>SNAMNDTPDDTFVSGYLLYLLAASSEEASAQFHDHIRAQGLRVPEWRVLACLVDNDAMMITRLA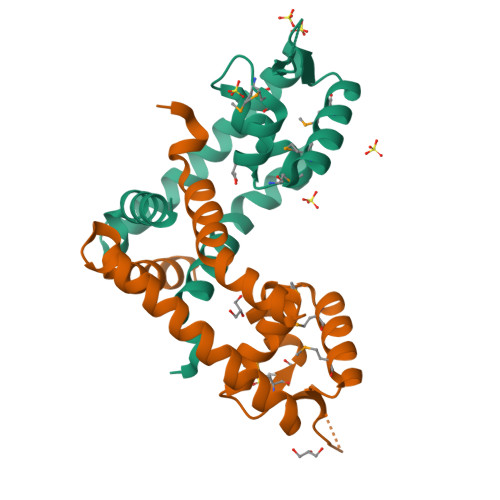KLSLMEQSRMTRIVDQMDARGLVTRVADAKDKRRVRVRLTDDGRALAESLVASARAHETRLLSALADTDAARIKGVLRTLLDVLDRPRESR[2x]>[3x]MERLRQIASQATAASA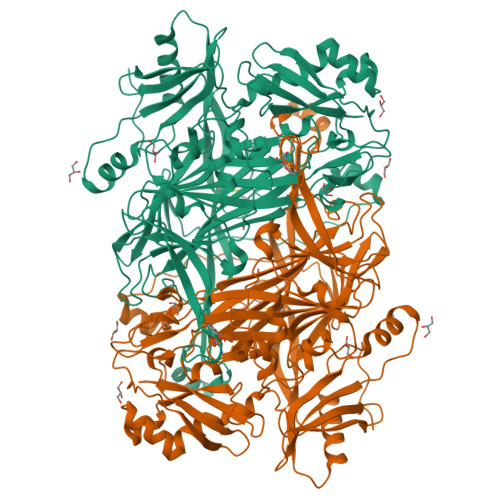APARPAHPLDPLSTAEIKAATNTVKSYFAGKKISFNTVTLREPARKAYIQWKEQGGPLPPRLAYYVILEAGKPGVKEGLVDLASLSVIETRALETVQPILTVEDLCSTEEVIRNDPAVIEQCVLSGIPANEMHKVYCDPWTIGYDERWGTGKRLQQALVYYRSDEDDSQYSHPLDFCPIVDTEEKKVIFIDIPNRRRKVSKHKHANFYPKHMIEKVGAMRPEAPPINVTQPEGVSFKMTGNVMEWSNFKFHIGFNYREGIVLSDVSYNDHGNVRPIFHRISLSEMIVPYGSPEFPHQRKHALDIGEYGAGYMTNPLSLGCDCKGVIHYLDAHFSDRAGDPITVKNAVCIHEEDDGLLFKHSDFRDNFATSLVTRATKLVVSQIFTAANYEYCLYWVFMQDGAIRLDIRLTGILNTYILGDDEEAGPWGTRVYPNVNAHNHQHLFSLRIDPRIDGDGNSAAACDAKSSPYPLGSPENMYGNAFYSEKTTFKTVKDSLTNYESATGRSWDIFNPNKVNPYSGKPPSYKLVSTQCPPLLAKEGSLVAKRAPWASHSVNVVPYKDNRLYPSGDHVPQWSGDGVRGMREWIGDGSENIDNTDILFFHTFGITHFPAPEDFPLMPAEPITLMLRPRHFFTENPGLDIQPSYAMTTSEAKRAVHKETKDKTSRLAFEGSCCGK>[2x]PQSQKILQFEDIMTNPFYRERFGTYMERIDKRALVGFWESAEHLKNANKSEIPQLVSE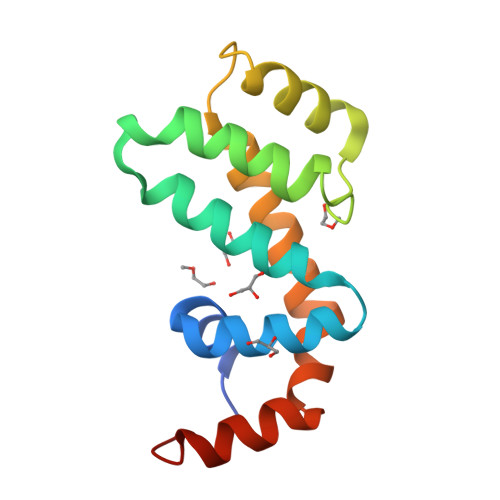MYQNFFVESKEISVEKSLYKEIQQCLVGNRGIEVFSKIQADVSEVLRERYYPSFLVSDLYEKLMRLEHHHHHH>[2x]GPNCAPGQKVKLFRASEPILSVLMWGVNHTINELSNVPVPVMLMPDDFKAYSKIKVDNHLFNKENLPSRFKFKEYCPMVFRNLRERFGIDDQDYQNSVTRSAP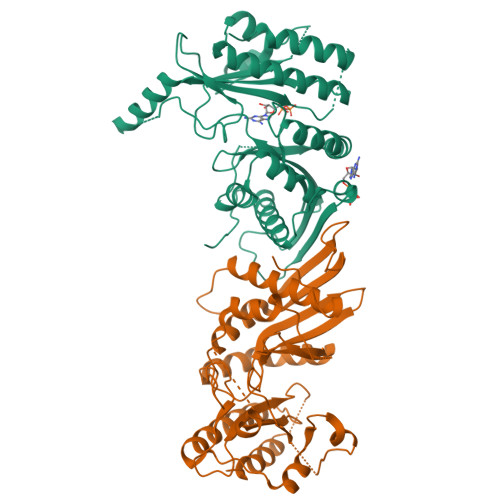INSDSQGRCGTRFLTTYDRRFVIKTVSSEDVAEMHNILKKYHQFIVECHGNTLLPQFLGMYRLTVDGVETYMVVMRNVFSHRLTVHRKYDLKGSTVAREASDKEKAKDLPTFKDNDFLNEGQKLHVGEESKKNFLEKLKRDVEFLAQLKIMDYSLLVGIHDVDRAEQEEMEVEERAEDEECENDGVGGNLLCSYGTPPDSPGNLLSFPRFFGPGEFDPSVDVYAMKSHESSPKKEVYFMAIIDILTPYDTKKKAAHAAKTVKHGAGAEISTVNPEQYSKRFNEFMSNILT> NPCIEVVPNITYQCMDQKLSKVPDDIPSSTKNIDLSFNPLKILKSYSFSNFSELQWLDLSRCEIETIEDKAWHGLHHLSNLILTGNPIQSFSPGSFSGLTSLENLVA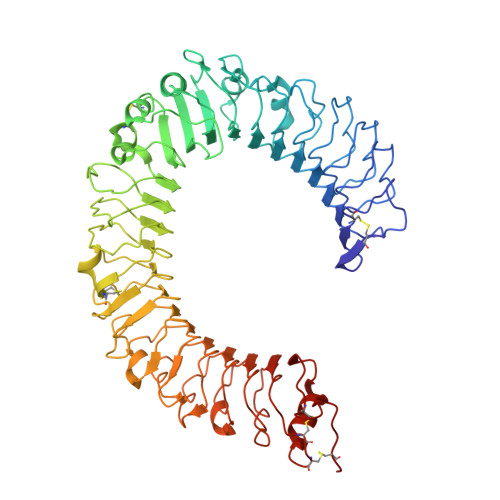VETKLASLESFPIGQLITLKKLNVAHNFIHSCKLPAYFSNLTNLVHVDLSYNYIQTITVNDLQFLRENPQVNLSLDMSLNPIDFIQDQAFQGIKLHELTLRGNFNSSNIMKTCLQNLAGLHVHRLILGEFKDERNLEIFEPSIMEGLCDVTIDEFRLTYTNDFSDDIVKFHCLANVSAMSLAGVSIKYLEDVPKHFKWQSLSIIRCQLKQFPTLDLPFLKSLTLTMNKGSISFKKVALPSLSYLDLSRNALSFSGCCSYSDLGTNSLRHLDLSFNGAIIMSANFMGLEELQHLDFQHSTLKRVTEFSAFLSLEKLLYLDISYTNTKIDFDGIFLGLTSLNTLKMAGNSFKDNTLSNVFANTTNLTFLDLSKCQLEQISWGVFDTLHRLQLLNMSHNNLLFLDSSHYNQLYSLKELALDTNQLKSVPDGIFDRLTSLQKIWLHTNPWDCSCPRIDYLSRWLNKNSQKEQGSAKCSGSGKPVRSIICPT> TSPQREATCTSEVSGCPKIYNPVCGTDGITYSNECVLCSE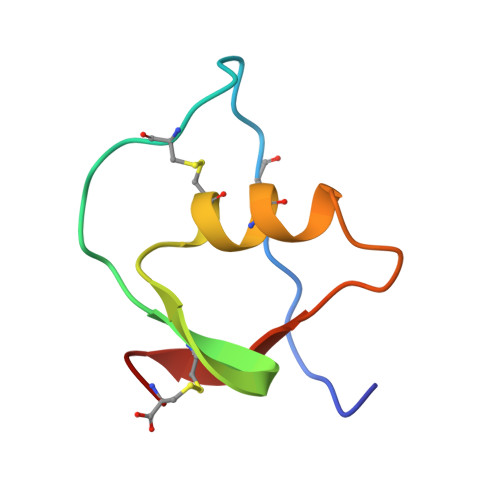NKKRQTPVLIQKSGPC> ISRLGPDSDFLTSVVAKASTSIVTPADRILVKQPLSASSFPGTRITGLSSYWERYKWLSAVARYVPAVPNTVACQFVMYIDTDPLDDPSNISDDNQIVRQAVSQAGSNQFNFNTSKTVPLIVRADNQYYYTGVDKQNLRFSLQGILYIIQVTDLINFNGELITQDLTCGSLFLDWLVNFSIPQIN

A major factor that limits the expansion of shrimp cultures is, however, infectious diseases from viruses, such as P. vannamei nodavirus (PvNV) and M. rosenbergii nodavirus (MrNV), which have inflicted heavy economic losses. The Nodaviridae genome comprises two single-stranded positive-sense RNA that encode the capsid protein for viral capsid assembly, the RNA polymerase for RNA replication, and the B2 protein for host RNA interference suppressor. While the shell domains (S-domains) of PvNV and MrNV contain conserved sequences of 62% identity, the protrusion domains (P-domains) and N-arms show low sequence identities of only 17% and 43%, respectively. In this work, we have determined the cryo-EM structures of T = 3 and T = 1 PvNV-LPs at atomic resolution, the crystal structures of the P-domains of PvNV and MrNV (PvNVPd and MrNVPd), and the crystal structure of the S-domain of PvNV (ΔN-ARM-PvNVSd) in the T = 1 subviral particle (SVP).

To examine whether or not the shrimp nodavirus capsid proteins could assemble into distinct particles in the absence of N-ARM, the crystal structure of the truncated PvNVSd (ΔN-ARM-PvNVSd, residues 38–250) was determined at resolution 3.1 Å and showed a T = 1 SVP architecture. In the final atomic model, the ΔN-ARM-PvNVSd comprising residues 66–250, without the disordered N-terminal region (38–65), organizes into the prevalent jelly-roll β-barrel fold with adjacent eight antiparallel β-strands. The T = 1 ΔN-ARM-PvNVSd SVP contains 120 Ca2+ ions occupying the Ca2+-binding sites at the interface of each subunit, which are conserved with the T = 3 PvNV-LP. In support of the conclusion that N-ARM serves as a molecular switch to control particle sizes, the negative-staining EM image of the ΔN-ARM-PvNV SVP (residues 45–368) was also recorded. The EM image showed that the ΔN-ARM-PvNV indeed form a T = 1 capsid of diameter ~24 nm consistent with T = 1 PvNV-LP. In addition, our two PvNV capsid protein deletion mutants both assemble into T = 1 SVPs, suggesting that a deletion of the N-ARM seems sufficient to produce a T = 1 capsid. Our recombinant PvNV capsid proteins assembled in vitro into three PvNV-LP categories, i.e., T = 3 PvNV-LP, T = 1 PvNV-LP, T = 1 ΔN-ARM-PvNV SVP and T = 1 ΔN-ARM-PvNVSd SVP, with corresponding diameters 350, 240, and 190 Å, respectively.> SHMILKLKHYNEQQSLYSKAIRWDFVIENTGNSYIDLRNVKVRYYFKDDYKNINFA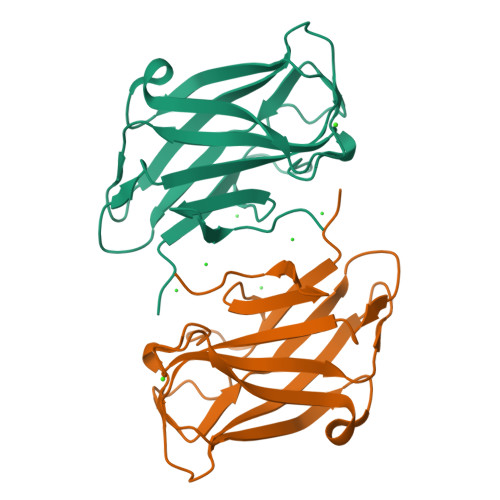VYFYSLGDEKNDVKGKVYNIRQSDSSHKYLEVTFEKGSIPPGDAAWVFGAITRDDWTEFNQEDDWSFLQGNSTFSYWDKMTVYISDKLVWGIEPY> XAH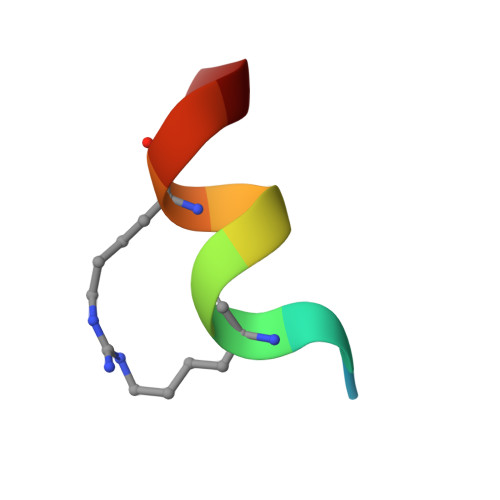LILHRLLA>MRVGIPTETKNNEFRVAITPAGVAELTRRGHEVLIQAGAGEGSAITDADFKAAGAQLVGTADQVWADADLLLKVKEPIAAEYGRLRHGQILFTFLHLAASRACTDALLDSGTTSIAYETVQTADGALPLLAPMSEVAGRLAAQVGAYHLMRTQGGRGVLMGGVPGVEPADVVVIGAGTAGYNAARIANGMGATVTVLDINIDKLRQLDAEFCGRIHTRYSSAYELEGAVKRADLVIGAVLVPGAKAPKLVSNSLVAHMKPGAVLVDIAIDQGGCFEGSRPTTYDHPTFAVHDTLFYCVANMP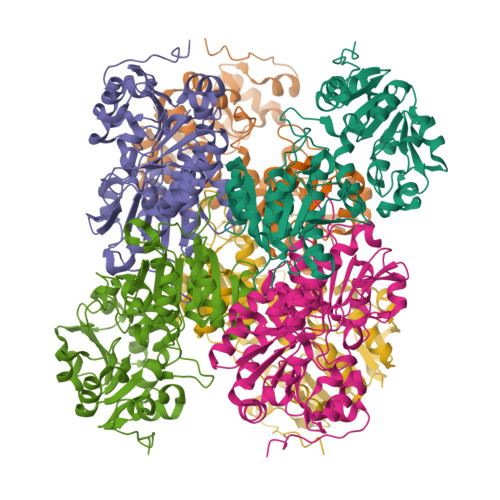ASVPKTSTYALTNATMPYVLELADHGWRAACRSNPALAKGLSTHEGALLSERVATDLGVPFTEPASVLA[6x]> MRFETLLKRAAQVGALVLLPLAAHAQEASAVDPARVDAVVKTSFTKLPEGWESRLQQDETQRICSVTRNNPSPEQAAAIMKAEEVRIKFPAGPVLGSWKDGAKVAQNGRGGQFSDPPGTVSGGNCYACHQLDPKEVSYGTLGPSLVGYGRERNFSAEDAKIAFAKVYDAQASLACSSMPRFGVNGVLTEQQIKDVVAYLFDPESPVN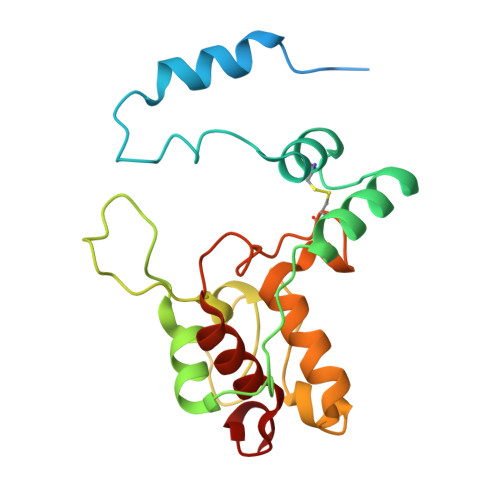K>MKNIKKNQVMNLGPNSKLLKEYKSQLIELNIEQFEAGIGLILGDAYIRSRDEGKTYCMQFEWKNKAYMDHVCLLYDQWVLSPPHKKERVNHLGNLVITWGAQTFKHQAFNKLANLFIVNNKKTIPNNLVENYLTPMSLAYWFM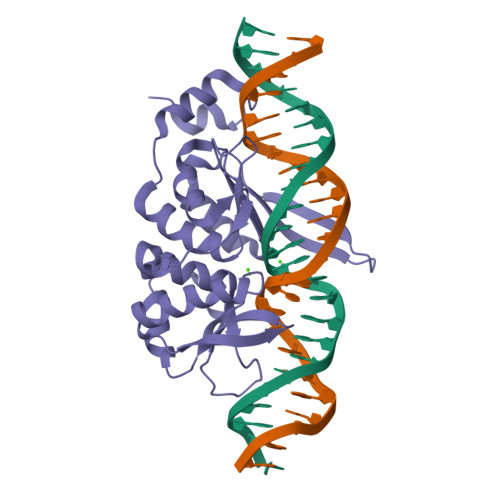DDGGKWDYNKNSTNKSIVLNTQSFTFEEVEYLVKGLRNKFQLNCYVKINKNKPIIYIDSMSYLIFYNLIKPYLIPQMMYKLPNTISSETFLK[2x]Computational design of KE07 involved construction of a theozyme to catalyze the chemical reaction, which was then grafted into the scaffold of imidazole glycerol phosphate synthase (HisF) from Thermotoga maritima. Catalytically essential residues from the initial design include a base (Glu101) that facilitates C−H bond cleavage, an H-bond donor (Lys222) to stabilize the phenoxide intermediate, and a π-stacking residue (Trp50), which was designed to stabilize the transition state and favor substrate binding through interactions with the aromatic ring of the substrate. This initial KE07 design (Round 1; R1) catalyzes the cleavage of 5-nitrobenzisoxazole, with 103-fold rate acceleration over the noncatalyzed reaction and a turnover rate (kcat) of 0.018 s−1.

Thus, the mechanism by which the remote mutations that appear in R5 and R6 increase activity is qualitatively different. This is mirrored in their location within the protein; in contrast to the initial mutations that affect the active site directly, the mutations in R5 (Val12Met) and R6 (Lys146Thr) are remote from the active site. The Val12Met and Phe77Ile mutations, also in the second shell, cause changes to internal cavities that cause a slight rotation in the backbone at Trp50 that also favors the alternative configuration. To the solution sampling of these states, we used HREX-MD simulations, which are among the most comprehensive computational methods to investigate conformational sampling. These results were consistent with the crystallography and kinetic analysis: whereas in R1 (original design), configuration A was the dominant substate that was sampled, by R5 we observe increased sampling of configurations B and C. By R7 and R7-2, configuration C (which was the only state we saw associated with product in the crystal structures) becomes the dominant substate sampled, with configurations A and B sampled only rarely. These simulations also reveal that the mobility of Glu101 was reduced as a result of the hydrogen bond formed to the indole nitrogen of Trp50 in R5; this could account for the improved pre-exponential factor from R5 onwards.

> MALAKRIDAALIMKDGRVVKGSNFENLRDSGDPVELGKFYSEIGIDELSFWDITASVEKRKTMLELVEKVAEQIDIPFTVGGGIHDFETASELILRGADKVEINTAAVENPSLITQIAQTFGSQAVVVYIAAKRVDGEFMVFTYSGKKNTGILLRDWVVEVEKRGAGEIVLGSIDRLGTKSGYDTEMIRFVRPLTTLPIIAHRGAGKMEHFLEAFLAGADAAKADSVFHFREIDVRELKEYLKKHGVNVRLE> GADHVFNIFKDLPDHKILEDKHYPAWLFTLDKPEKTYGELAMT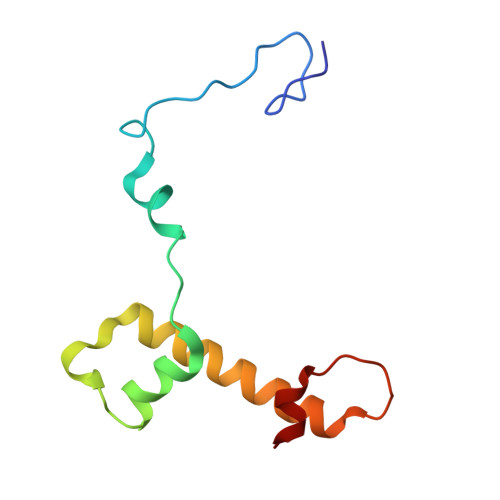FLYGVGIENATLDEYLRFTRLHTKNLIKLNNMRLKKSKRSSVKPLFWDA ethyl {3-[4-amino-5-{3-[(cyclopropylsulfonyl)amino]prop-1-yn-1-yl}-2-oxopyrimidin-1(2H)-yl]oxetan-3-yl}acetate 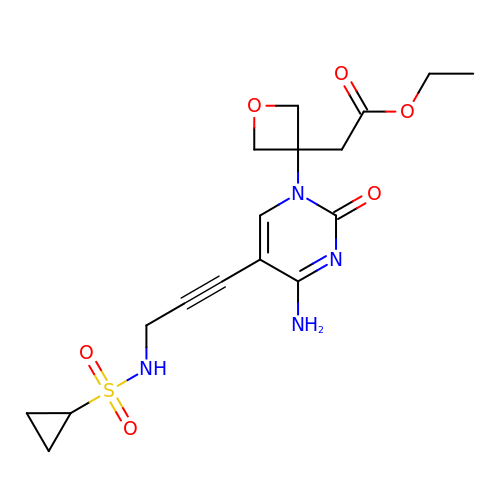| C17 H22 N4 O6 S | MIAWQMZUJQYSPX-UHFFFAOYSA-N>[10x]GASKAFYSAGDKLFQPGDDAVASMQTYSVAQFLQPFTLNPAKASSDYLGKWVKVRGVIVDIRRKSGIAGSYYFIVTMRDEQNKTDKRLTFNFGSHNSADVEALSNGSVATIVGQVHQVQDSTIPTLQNPKVVK

KPN03535 (gi|152972051) is a putative lipoprotein of unknown function that is secreted by Klebsiella pneumoniae MGH 78578. The crystal structure reveals that despite a lack of any detectable sequence similarity to known structures, it is a novel variant of the OB-fold and structurally similar to the bacterial Cpx-pathway protein NlpE, single-stranded DNA-binding (SSB) proteins and toxins. The N-terminus of KPN03535 has a lipoprotein signature, indicated by the presence of an LSGC motif, as well as predictions from LipoP 1.0. In conclusion, the crystal structure of KPN03535 reveals a novel divergent member of the prevalent OB-fold and suggests that it is most likely to be a nucleic acid-binding protein.

The crystallized protein is comprised of a glycine left after cleavage of the expression and purification tag followed by KPN03535 residues 23–154. The final model contains ten monomers (chains A–J), two PEG molecules (PEG 600 fragments from the crystallization solution) and 323 water molecules in the asymmetric unit. The ten monomers are almost identical in structure and completeness and superimpose extremely well, with pairwise r.m.s.d. values ranging from only 0.2 to 0.4 Å. Residues 36–69 constitute three additional α-helices (α−2, α−1 and α0) which are not observed in other structures of the same fold. The capping helix α in KPN03535 is shorter than in the toxins and NlpE, although it is similar to that observed in BOF protein. In the crystal structure, the protein assembles as two stacked pentameric rings, formed by loose interdigitation of the ‘finger-like’ β1–L12–β2 structure, with outer and inner diameters of ∼80 Å and ∼40 Å, respectively, and a thickness of ∼40 Å. The buried surface area of each monomer within each pentamer (∼540 Å2) and each monomer in the interface between the two pentamers (∼600 Å2) is low. The quaternary structure analysis does not suggest sufficiently strong and extensive interactions to enable complex formation in solution, suggesting that these pentamers could be a crystallization artifact. Crystal-packing and assembly analysis using PISA supported by analytical size-exclusion chromatography and static light scattering suggest that a monomer is the likely oligomeric state. Analysis of the electrostatic surface potential indicates that KPN03535 most closely resembles PriB and aspartyl-tRNA synthetase, with a prominent positively charged area similar to the DNA-binding region of these two proteins.>MRGSHHHHHHRSPSKVQELSVYEINELDRHSPKILKNAFSLMFGLGDLVPFTNKLYTGDLKKRVGITAGLCVVIEHVPEKKGERFEATYSFYFGDYGHLSVQGPYLTYEDSFLAITGGAGIFEGAYGQVKLQQLVYPTKLFYTFYLK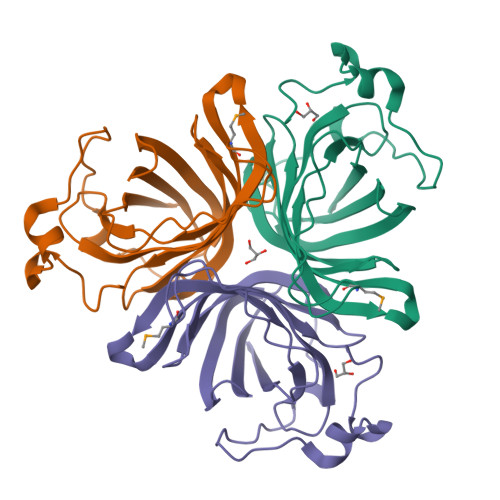GLANDLPLELTGTPVPPSKDIEPAPEAKALEPSGVISNYTN[3x]There have been increased efforts recently to “drug” RNA using orally bioavailable, low-molecular-weight compounds. This study combines two of the most powerful tools of modern drug discovery, high-throughput screening and structure-based design, to target the theophylline aptamer, a tertiary-structured RNA that binds theophylline with high affinity and selectivity. That structure revealed how multiple interdependent components of the RNA form a well-defined ligand binding pocket that enables theophylline to bind with submicromolar affinity while excluding closely related compounds such as caffeine (which differs by a single methyl group) by more than 10,000-fold. Previous biophysical and modeling studies have shown that the aptamer undergoes a large conformational rearrangement upon binding theophylline. X-ray crystal structures were determined for the aptamer, both in isolation and in complex with various ligands, revealing the molecular basis for ligand binding.

The Kd value for theophylline was 0.67 µM, which is in good agreement with the previously reported value. The second strategy involved replacing the G2–U32 wobble pair at the base of the RNA aptamer by a G–C Watson–Crick pair, thus stabilizing the corresponding stem. Thus, to reveal atomic-level details of the RNA–ligand interaction, it was necessary to turn to the second crystallization strategy, with the stabilized aptamer stem and no protein component. This approach gave high-quality crystals (1.42–2.70 Å resolution) for the various aptamer–ligand complexes. The previous NMR structure of the theophylline-bound aptamer was used to provide phasing information to solve the structure of these five complexes. The X-ray crystal structure of the aptamer–theophylline complex reveals a Mg2+ ion bound to N7 of G25 and coordinated to five water molecules, which stabilizes the S-turn that shapes the ligand binding site. Two Na+ ions assist in stabilizing this structure: the first coordinates to N7 of A5, O4 of U6, and the 2′-hydroxyl of C22; the second coordinates to both O2 and the 2′-hydroxyl of U23 and forms water-mediated hydrogen bonding interactions with the sugar-phosphate of U24 and the phosphate of A28. The structural data also revealed how three bound cations help to stabilize the binding pocket by coordinating to multiple residues of the RNA.

>[2x]GGCGAUACCAGCCGAAAGGCCCUUGGCAGCGCC>MVYYPKKYELYKADEVPTEVVETDILIIGGGFSGCGAAYEAAYWAKLGGLKVTLVEKAAVERSGAVAQGLSAINTYIDLTGRSERQNTLEDYVRYVTLDMMGLAREDLVADYARHVDGTVHLFEKWGLPIWKTPDGKYVREGQWQIMIHGESYKPIIAEAAKMAVGEENIYERVFIFELLKDKNDPNAVAGAVGFSVREPKFYVFKAKAVILATGGATLLFRPRSTGEAAGRTWYAIFDTGSGYYMGLKAGAMLTQFEHRFIPFRFKDGYGPVGAWFLFFKCKAKNAYGEEYIKTRAAELEKYKPYGAAQPIPTPLRNHQVMLEIMDGNQPIYMHTEEALAELAGGDKKKLKHIYEEAFEDFLDMTVSQALLWACQNIDPQEQPSEAAPAEPYIMGSHSGEAGFWVCGPEDLMPEEYAKLFPLKYNRMTTVKGLFAIGDCAGANPHKFSSGSFTEGRIAAKAAVRFILEQKPNPEIDDAVVEELKKKAYAPMERFMQYKDLSTADDVNPEYILPWQGLVRLQKIMDEYAAGIATIYKTNEKMLQRALELLAFLKEDLEKLAARDLHELMRAWELVHRVWTAEAHVRHMLFRKETRWPGYYYRTDYPELNDEEWKCFVCSKYDAEKDEWTFEKVPYVQVIEWSF[2x];>[2x]MPSFVNPEKCDGCKALERTACEYICPNDLMTLDKEKMKAYNREPDMCWECYSCVKMCPQGAIDVR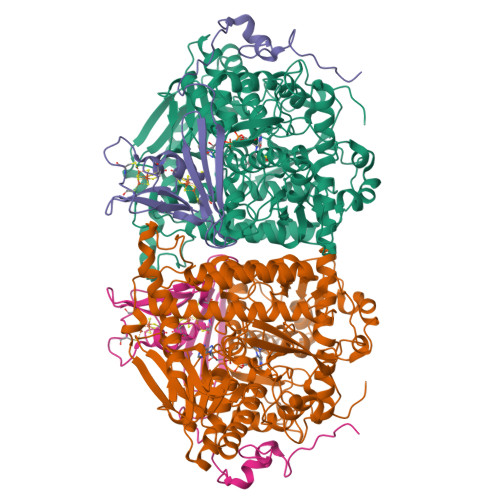GYVDYSPLGGACVPMRGTSDIMWTVKYRNGKVLRFKFAIRTTPWGSIQPFEGFPEPTEEALKSELLAGEPEIIGTSEFPQVKKKA> GSHMASHLDGVPEGGIDFTPHNGTKKIINTVAEVNKLSDASGSSIHSHLTNNALVEIHTANGRWVRDIYLPQGPDLEGKMVR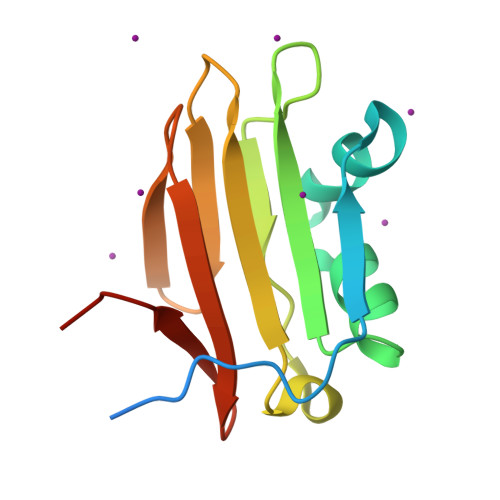FVSSAGYSSTVFYGDRKVTLSVGNTLLFKYVNGQWFRSGELENN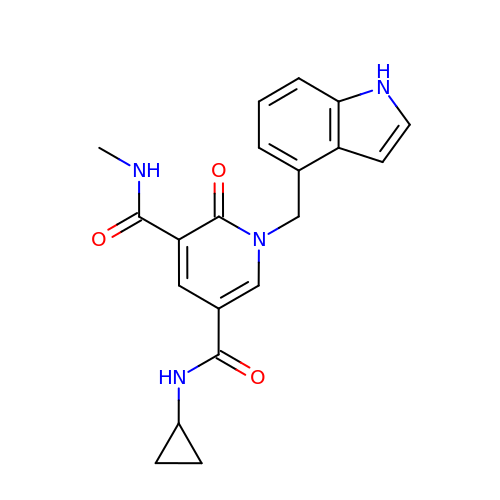~{N}5-cyclopropyl-1-(1~{H}-indol-4-ylmethyl)-~{N}3-methyl-2-oxidanylidene-pyridine-3,5-dicarboxamide | C20 H20 N4 O3 | PDCBJZVPIGAEBL-UHFFFAOYSA-N> TDPRAKWVPQDNDIQACDYWRHCSIDGNICDCSGGSLTNCPPGTKLATASWVASCYNPTDGQS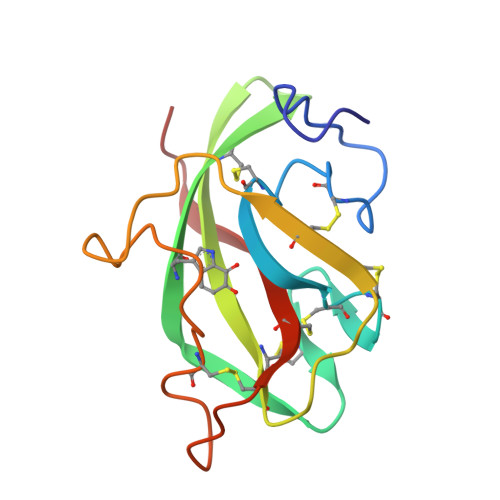YLIAYRDCCGYNVSGRCPCLNTEGELPVYRPEFANDIIWCFGAEDDAMTYHCTISPIVGKAS In Vaccinia virus (VACV), copies of the double-jelly-roll protein D13 bind to the viral membrane via interaction with its partner protein A17 and assemble into a scaffold surrounding the viral membrane. This process leads to the formation of a spherical immature virion (IV). The 62-kDa D13 protein exists as trimers both in vivo and in vitro, and structures of the recombinantly expressed D13 trimer have been determined by X-ray crystallography. D13 adopts a double-jelly-roll structure composed of 8 antiparallel β-strands.

We purified recombinant D13 trimer protein for structure determination using single-particle cryo-electron microscopy (cryo-EM). Initial attempts were hampered by problems associated with preferred particle orientation and spontaneous protein assembly into honeycomb-like crystalline patches that consist of rings of five or six trimers. This problem was mitigated using holey EM grids coated with a graphene oxide support film, and the cryo-EM structure of the D13 trimer was determined at 2.3 Å resolution. The refined atomic model based on this structure was largely identical to previously reported crystal structures (average RMSD 0.495 Å). However, the presence of the short N-terminal tail α-helix (aa 1-10) was inconsistent with previously reported models. Our cryo-EM map showed intact N-terminal tail α-helices in all three subunits, with or without imposition of 3-fold symmetry, although reduced local map resolution and the increased B-factor suggested that the helix was prone to dislocation. In our structure, the hydrophobic face of the N-terminal helix (M1, I5, I6 and L9) was held in a pocket of surrounding hydrophobic residues from the adjacent subunits. Additional hydrogen bonds were identified between the side chains of T4, N2, Q35 and the carboxylic groups of V451, L452, and N2. The protein solution turned turbid after dialysis into low-salt buffer, but examination by transmission electron microscopy (TEM) showed aggregated honeycomb-like patches and rodlets without any IV-like particles. We found that the N-terminal short tail α-helix of D13 is critical for in vitro assembly into ordered structures. We propose that repositioning of the N-terminal tail α-helix away from D13 toward the surface of the lipid bilayer may act as a molecular trigger that initiates scaffold assembly in vivo.

>AMNNTIINSLIGGDDSIKRSNVFAVDSQIPTLYMPQYISLSGVMTNDGPDNQAIASFEIRDQYITALNHLVLSLELPEVKGMGRFGYVPYVGYKCINHVSISSCNGVIWEIEGEELYNNCINNTIALKHSGYSSELNDISIGLTPNDTIKEPSTVYVYIKTPFDVEDTFSSLKLSDSKITVTVTFNPVSDIVIRDSSFDFETFNKEFVYVPELSFIGYMVKNVQIKPSFIEKPRRVIGQINQPTATVTEVHAATSLSVYTKPYYGNTDNKFISYPGYSQDEKDYIDAYVSRLLDDLVIVSDGPPTGYPESAEIVEVPEDGIVSIQDADVYVKIDNVPDNMSVYLHTNLLMFGTRKNSFIYNISKKFSAITGTYSDATKRTIFAHISHSINIIDTSIPVSLWTSQRNVYNGDNRSAESKAKDLFINDPFIKGIDFKNKTDIISRLEVRFGNDVLYSENGPISRIYNELLTKSNNGTRTLTFNFTPKIFFRPTTITANVSRGKDKLSVRVVYSTMDVNHPIYYVQKQLVVVCNDLYKVSYDQGVSITKIMG[3x]> IIGGTESKPHSRPYMAYLEIVTSNGPSKFCGGFLIRRNFVLTAAHCAGRSITVTL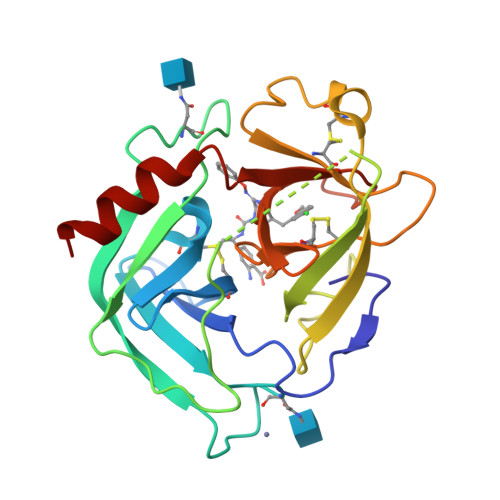GAHNITEEEDTWQKLEVIKQFRHPKYNTSTLHHDIMLLKLKEKASLTLAVGTLPFPSQKNFVPPGRMCRVAGWGRTGVLKPGSDTLQEVKLRLMDPQACSHFRDFDHNLQLCVGNPRKTKSAFKGDSGGPLLCAGVAQGIVSYGRSDAKPPAVFTRISHYRPWINQILQAN> MTQPASSRVVFDPSNPTTFSVEAIAAYTPVALIRLLNASGPLQPGHRVDIADARSIYTVGAAASAARARANHNANTIRRTAMFAETDP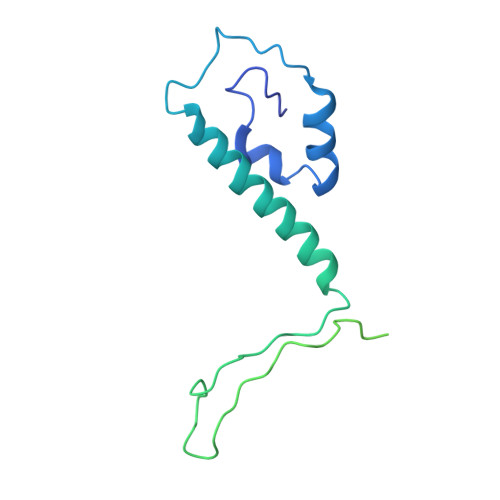MTWLRPTVGLKRTFNPRIIRPQPPNPSMSLGISGPTILPQKTQSADQSALQQPAALAFSGSSPQHPPPQTTSASVGQQQHVVSGSSGQQPQQGAQSSTVQPTTGSPPAAQGVPQSTPPPTQNTPQGGKGQTLSHTGQSGNASRSRRV>MGKGHHHHHHGSERTGTQPLGVQGLTEEQRMMIRELMDAQMKTFDTTFSHFKNFRLPGVLSSGCELPESLQAPSREEAAKWSQVRKDLCSLKVSLQLRGEDGSVWNYKPPADSGGKEIFSLLPHMADMSTYMFKGIISFAKVISYFRDLPIEDQISLLKGAAFELCQLRFNTVFNAETGTWECGRLSYCLEDTAGGFQQLLLEPMLKFHYMLKKLQLHEEEYVLMQAISLFSPDRPGVLQHRVVDQLQEQFAITLKSYIEC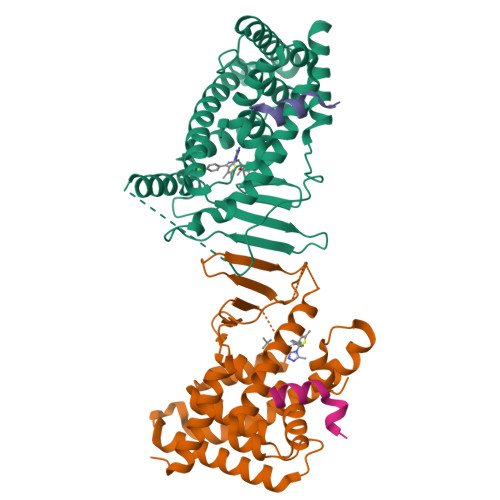NRPQPAHRFLFLKIMAMLTELRSINAQHTQRLLRIQDIHPFATPLMQELFGITGS[2x];>[2x]CPSSHSSLTERHKILHRLLQEGSPS>MVSKADNSA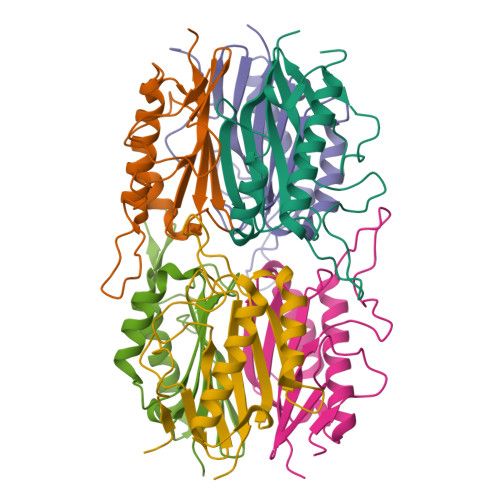KLVEGKAKPMGSFPHVKRAGDFLFVSGTSSRRPDNTFVGAEPDDTGRPRPNIELQTREVISNIRDILQSVGADLGDVVEVCSYLVNMNDFAAYNKVYAEFFDATGPARTTVAVHQLPHPQLVIEIKVVAYKPL[9x]>MAVILHPNETIFNDFCKKSTTCEVLKYNTCLGSPLPYTHTSLILAEDSETQEEAFEKLAMWSGLRNAPRCWAVIQPLLCAVYMPKCENGKVELPSQHLCQATRNPCSIVERERGWPNFLKCENKEQFPKGCQNEVQKLKFNTSGQCEAPLVKTDIQASWYKDVEGCGIQCDNPLFTEDEHSDMHKLEHHHHHH[2x]

Smo consists of an extracellular N-terminal region containing a cysteine rich domain (CRD), a heptahelical transmembrane segment (7TM) and an intracellular C-terminal tail (C-term). Smo belongs to the G-protein coupled receptor (GPCR) superfamily of proteins, most closely related to the Frizzled (Fz) group of Wnt receptors. In the absence of Hh ligands, Ptch1 inhibits the function of Smo, a 7-pass TM protein that is encoded by a human oncogene. Our work now shows that the Smo CRD in vertebrates binds to oxysterols and mediates the ability of these lipids to activate Hh signaling.

Although we set-up crystallization trials with the entire zSmo ectodomain (residues 29–212), the N- and C-terminal regions could not be traced due to missing electron density and thus were not included in the final model. The small interface between the two zSmo CRD molecules observed in the asymmetric unit of the crystal (buried surface area of 490 Å2) and a crystal contact formed by a zinc ion bonded to three different protein chains (one chain A and two chain B molecules) suggested that the dimeric arrangement observed in the crystal is not likely to be of functional significance. In agreement with this crystal packing analysis, purified zSmo ectodomain behaved as a monomer in solution at low concentration (5 µM) when assessed using multi angle light scattering. The zSmo CRD monomer adopts a globular fold composed of four α helices (α1: residues Q77-N92; α2: P94-Y108; α3: Q122-N130; α3′: S133-E138) and a short two-stranded β sheet (β1: K43-S45 and β2: K116-E118). Disulfide bridges I, II, III, and IV lock the four helices together into a tight bundle, whereas disulfide bridge *, formed by the N- and C-terminal cysteines, orients the termini in close proximity and away from the helical bundle. Structure-based evolutionary analysis of zSmo CRD revealed that the closest structural relatives are the CRDs of Frizzled 8 (Fz8; Dann et al., 2001; Janda et al., 2012), secreted Frizzled-related protein 3 (sFRP3, Dann et al., 2001) and muscle-specific kinase (MuSK, Stiegler et al., 2009), shown clustered in the blue branch in Figure 5B. To investigate the putative oxysterol binding site in the Smo CRD, we calculated the volumes of potential binding pockets in our zSmo CRD structure. The most prominent groove is indeed located at an equivalent position to the Fz8 palmitoleyl-binding groove. The residues forming this groove are highly conserved in all vertebrate Smo CRDs, and the volume (551 Å3) and shape of the groove is sufficient for 20(S)-OHC binding. Computational docking using AutoDock showed that the hydrophobic groove on the zSmo CRD surface can accommodate 20(S)-OHC with a favorable free energy of binding.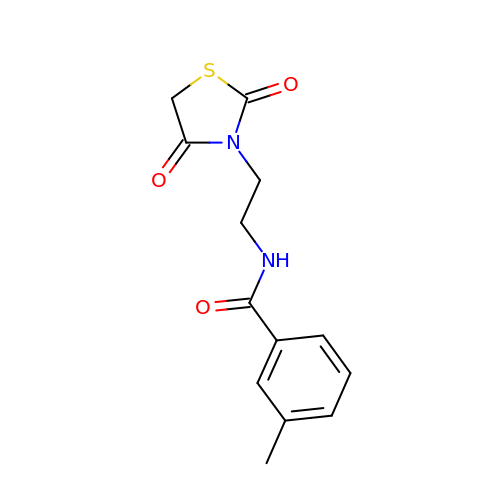N-(2-(2,4-dioxothiazolidin-3-yl)ethyl)-3-methylbenzamide | C13 H14 N2 O3 S | LNKJOLQQLIVVPE-UHFFFAOYSA-N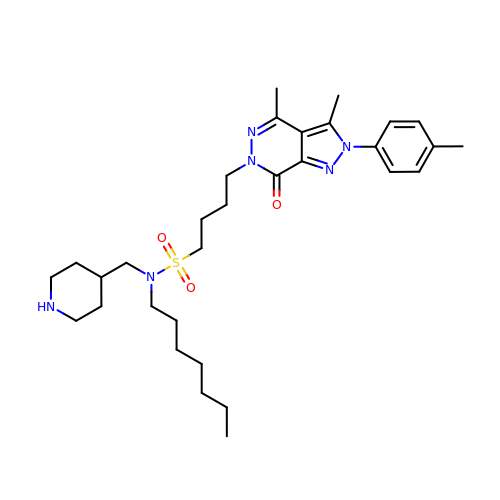4-[3,4-dimethyl-2-(4-methylphenyl)-7-oxidanylidene-pyrazolo[3,4-d]pyridazin-6-yl]-~{N}-heptyl-~{N}-(piperidin-4-ylmethyl)butane-1-sulfonamide | C31 H48 N6 O3 S | DVTXDCJEWQTSFM-UHFFFAOYSA-N(3Z)-6-(4-HYDROXY-3-METHOXYPHENYL)-3-(1H-PYRROL-2-YLMETHYLENE)-1,3-DIHYDRO-2H-INDOL-2-ONE | C20 H16 N2 O3 | 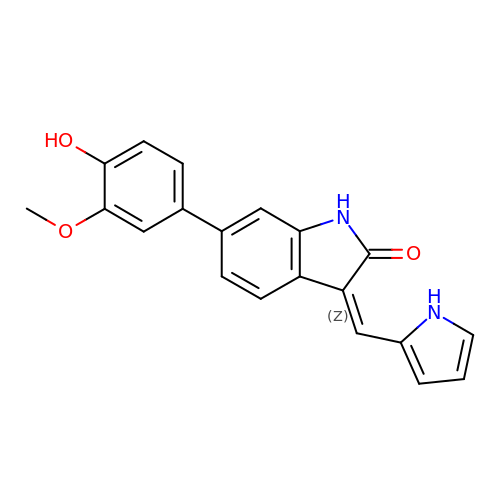AYSXURJZVXBSRV-WJDWOHSUSA-N>XFFGPQYQ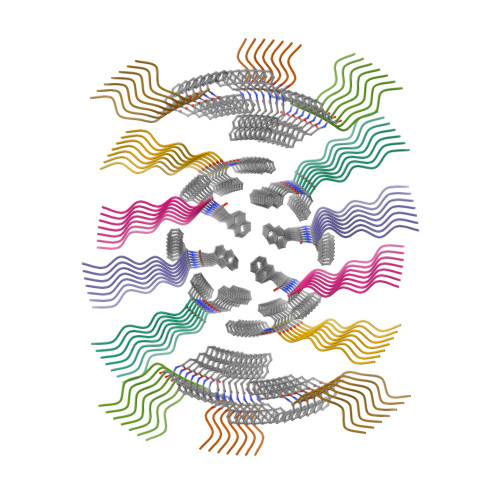P[7x]2'-DEOXYGUANOSINE-5'-DIPHOSPHATE | C10 H15 N5 O10 P2 | 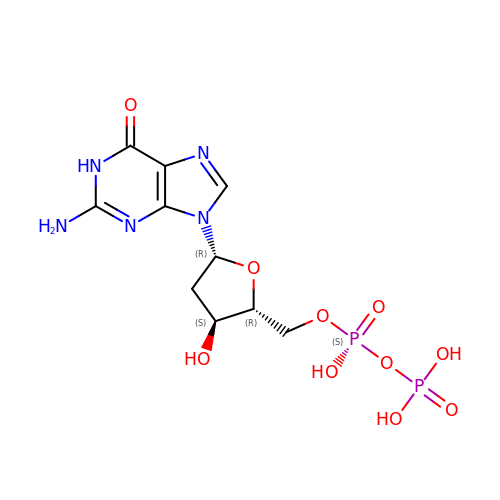CIKGWCTVFSRMJU-KVQBGUIXSA-N>[2x]DLYDDDDKDPTLMKISRGLLKTILEA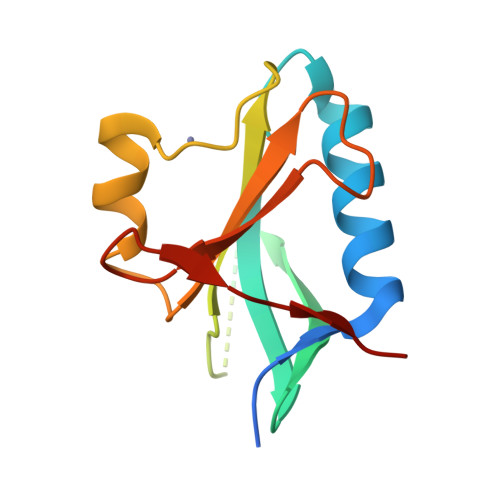AKSAHPDEFIALLSGSKDVMDELIFLPFVSGSVSAVIHLDMLPIGMKVFGTVHSHPSPSCRPSEEDLSLFTRFGKYHIIVCYPYDENSWKCYNRKGEEVELEVVEKD> GPGYQDPGNIQIQSMPKVKERVSVPSKDDTIYSYHDSIKDSIKAVVNISTEKKIKNNFIGGGVFNDPFFQQFFGDLGGMIPKERMERALGSGVIISKDGYIVTNNHVIDGADKIKVTIPGSNKEYSATLVGTDSESDLAVIRITKDNLPTIKFSDSNDISVGDLVFAIGNPFGVGESVTQGIVSALNKSGIGINSYENFIQTDASINPGNSGGALIDSRGGLVGINTAIISK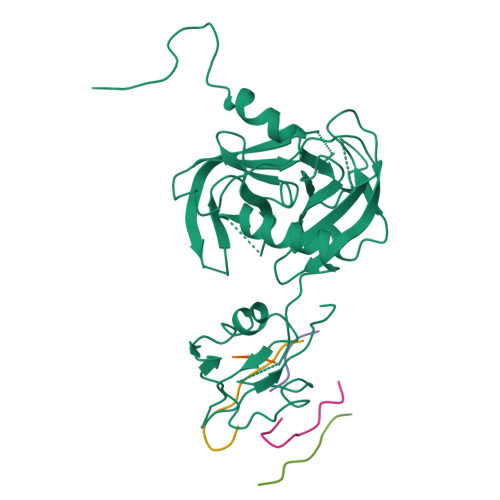TGGNHGIGFAIPSNMVKDTVTQLIKTGKIERGYLGVGLQDLSGDLQNSYDNKEGAVVISVEKDSPAKKAGILVWDLITEVNGKKVKNTNELRNLIGSMLPNQRVTLKVIRDKKERAFTLTLAERKNPNKKETISAQNGAQGQLNGLQVEDLTQETKRSMRLSDDVQGVLVSQVNENSPAEQAGFRQGNIITKIEEVEVKSVADFNHALEKYKGKPKRFLVLDLNQGYRIILVK;> AAA;> AAAAA;> AAKAAAAAAA;> AAAAAAAA;> AAAAAAAAAAA>AVYNIGWSFNVNGARGKSFRAGDVLVFKYIKGQHNVVAVNGRGYASCSAPRGARTYSSGQDRIKLTRGQNYFICSFP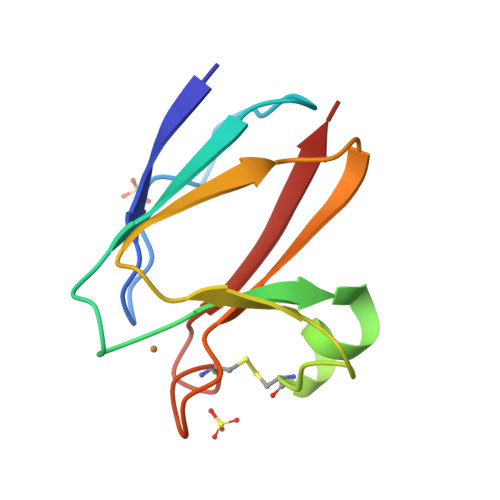GHCGGGMKIAINAK[3x]> MVKKMVIAVRKDLDMGKGKIAAQVAHAAVTCAIRSMKINRDVFNEWYDEGQRKIVVK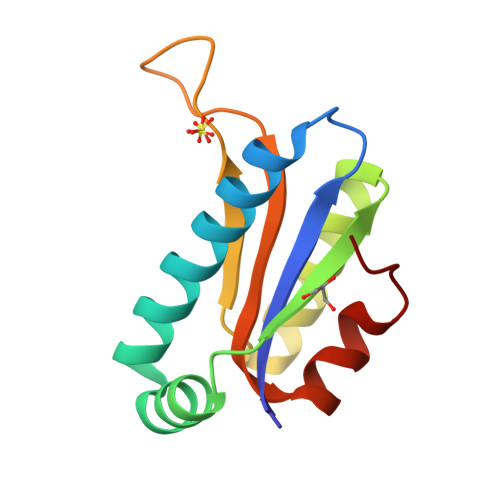VNDLDEIMEIKRMADSMGIVNEIVQDRGYTQVEPGTITCIGLGPDEEEKLDKITGKYKLL>GPLGSMSEEQVAQDTEEVFRSYVFYRHQQEQEAEGVAAPADPEMVTLPLQPSSTMGQVGRQLAIIGDDINRRYDSEFQTMLQHLQPTAENAYEYFTKIATSLFESGINWGRVVALLGFGYRLALHVYQHGLTGFLGQVTRFVVDFMLHHSIA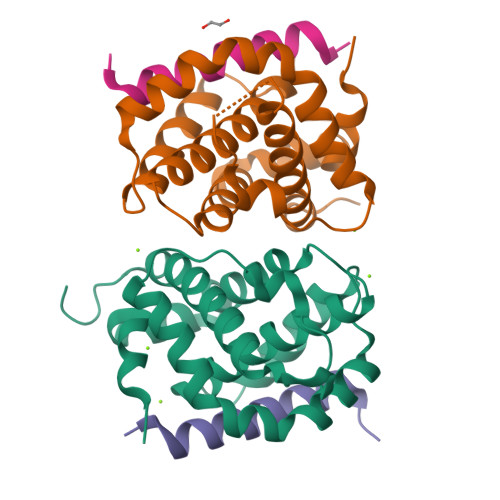RWIAQRGGWVAALNLGNG[2x];>DMRPEIRIAQELRRXGDEFNATYARR[2x]> PVQLSKEQEELIRTLLGAHTRHMGTMFEQFVQFRPPAHLFIHHQPLPTLAPVLPLVTHFADINTFMVLQVIKFTKDLPVFRSLPIEDQISLLKGAAVEICHIVLNTTFCLQTQNFLCGPLRYTIEDGARVGFQVEFLELLFHFHGTLRKLQLQEPEYVLLAAMALFSPDRPGVTQR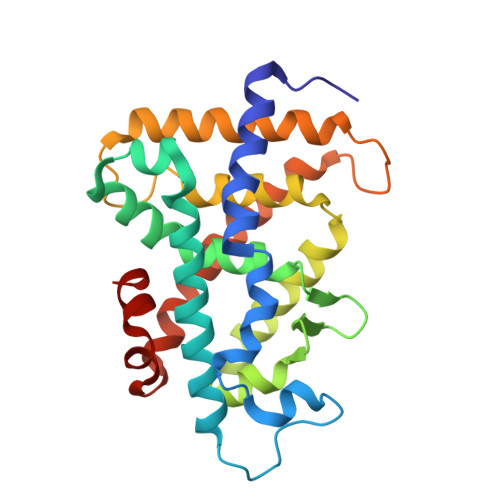DEIDQLQEEMALTLQSYIKGQQRRPRDRFLYAKLLGLLAELRSINEAYGYQIQHIQGLSAMMPLLQEICS> MFCFQCQETAKNTGCTVKGMCGKPEETANLQDLLIFVLRGIAIYGEKLKELGQPDRSNDDFVLQGLFATITNANWDDARFEAMISEGLARRDKLR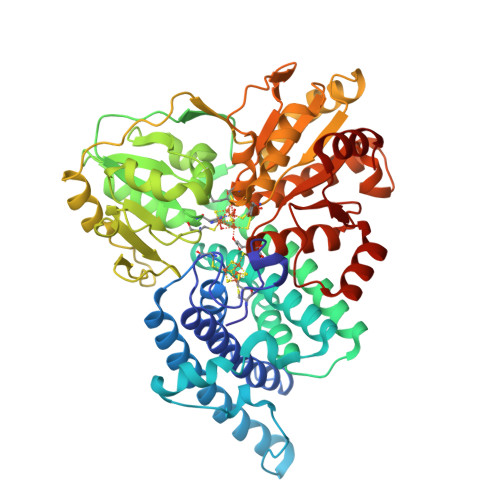NAFLAVYKAKNGKDFSEPLPEAATWTGDSTAFAEKAKSVGILATENEDVRSLRELLIIGLKGVAAYAEHAAVLGFRKTEIDEFMLEALASTTKDLSVDEMVALVMKAGGMAVTTMALLDEANTTTYGNPEITQVNIGVGKNPGILISGHDLKDMAELLKQTEGTGVDVYTHGEMLPANYYPAFKKYPHFVGNYGGSWWQQNPEFESFNGPILLTTNCLVPLKKENTYLDRLYTTGVVGYEGAKHIADRPAGGAKDFSALIAQAKKCPPPVEIETGSIVGGFAHHQVLALADKVVEAVKSGAIKRFVVMAGCDGRQKSRSYYTEVAENLPKDTVILTAGCAKYRYNKLNLGDIGGIPRVLDAGQCNDSYSLAVIALKLKEVFGLDDINDLPVSYDIAWYEQKAVAVLLALLFLGVKGIRLGPTLPAFLSPNVAKVLVENFNIKPIGTVQDDIAAMMAGK>AKPDRSSFVPSLFSKKKKNVTMRSIKTTRDRVPTYQYNMNFEKLGKCIIINNKNFDKVTGMGVRNGTDKDAEALFKCFRSLGFDVIVYNDCSCAKMQDLLKKASEEDHTNAACFACILLSHGEENVIYGKDGVTPIKDLTAHFRGDRCKTLLEKPKLFFIQACRGTELDDGIQ[2x];>ANPRYKIPVEADFLFAYSTVPGYYSWRSPGRGSWFVQALCSILEEHGKDLEIMQILTRVNDRVARHFESQSDDPHFHEKKQIPCV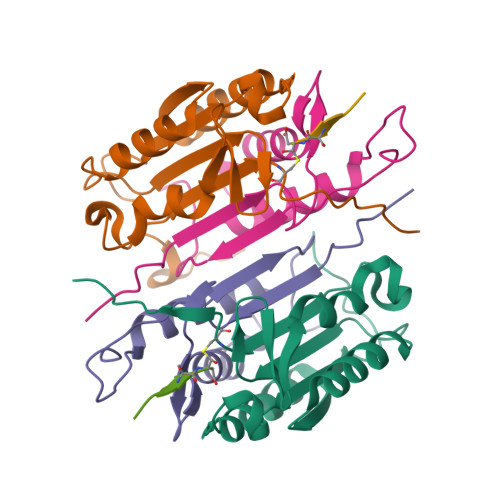VSMLTKELYFSQ[2x]Nitrogenase catalyzes the ATP-dependent reduction of dinitrogen to ammonia during the process of biological nitrogen fixation that is essential for sustaining life. The Fe-protein mediates ATP-dependent electron transfer (ET) through its [4Fe:4S] cluster to the intermediate [8Fe:7S] P-cluster in the MoFe-protein; the electrons are subsequently shuttled to a [7Fe:1Mo:9S:1C]-R-homocitrate metallocluster, the FeMo-cofactor, within the active site of the MoFe-protein. The active site FeMo-cofactor contains a [7Fe:1Mo:9S:1C] metallocluster coordinated with an R-homocitrate (HCA) molecule.

Indeed, the determination of intact MoFe-protein structures required either surfactants or the use of carbon-layered grids, due to the localization of MoFeAs-isolated to the air AWI, causing strong orientation bias, and disorder of its α-subunit. The use of cryo-electron-tomography (cryoET) was crucial for the validation of the MoFe-protein grid and freezing conditions. Optimized vitrification of the as-isolated MoFe-protein alone (MoFeAs-isolated) yielded a 2.13 Å resolution structure in the presence of detergent.

>MTGMSREEVESLIQEVLEVYPEKARKDRNKHLAVNDPAVTQSKKCIISNKKSQPGLMTIRGCAYAGSKGVVWGPIKDMIHISHGPVGCGQYSRAGRRNYYIGTTGVNAFVTMNFTSDFQEKDIVFGGDKKLAKLIDEVETLFPLNKGISVQSECPIGLIGDDIESVSKVKGAELSKTIVPVRCEGFRGVSQSLGHHIANDAVRDWVLGKRDEDTTFASTPYDVAIIGDYNIGGDAWSSRILLEEMGLRCVAQWSGDGSISEIELTPKVKLNLVHCYRSMNYISRHMEEKYGIPWMEYNFFGPTKTIESLRAIAAKFDESIQKKCEEVIAKYKPEWEAVVAKYRPRLEGKRVMLYIGGLRPRHVIGAYEDLGMEVVGTGYEFAHNDDYDRTMKEMGDSTLLYDDVTGYEFEEFVKRIKPDLIGSGIKEKFIFQKMGIPFREMHSWDYSGPYHGFDGFAIFARDMDMTLNNPCWKKLQAPWE[2x];>[2x]SQQVDKIKASYPLFLDQDYKDMLAKKRDGFEEKYPQDKIDEVFQWTTTKEYQELNFQREALTVNPAKACQPLGAVLCALGFEKTMPYVHGSQGCVAYFRSYFNRHFREPVSCVSDSMTEDAAVFGGQQNMKDGLQNCKATYKPDMIAVSTTCMAEVIGDDLNAFINNSKKEGFIPDEFPVPFAHTPSFVGSHVTGWDNMFEGIARYFTLKSMDDKVVGSNKKINIVPGFETYLGNFRVIKRMLSEMGVGYSLLSDPEEVLDTPADGQFRMYAGGTTQEEMKDAPNALNTVLLQPWHLEKTKKFVEGTWKHEVPKLNIPMGLDWTDEFLMKVSEISGQPIPASLTKERGRLVDMMTDSHTWLHGKRFALWGDPDFVMGLVKFLLELGCEPVHILCHNGNKRWKKAVDAILAASPYGKNATVYIGKDLWHLRSLVFTDKPDFMIGNSYGKFIQRDTLHKGKEFEVPLIRIGFPIFDRHHLHRSTTLGYEGAMQILTTLVNSILERLDEETRGMQATDYNHDLVR> RICFNHQSSQPQTTKTCSPGES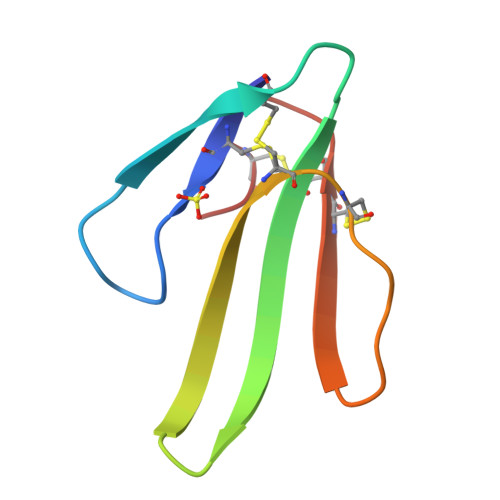SCYHKQWSDFRGTIIERGCGCPTVKPGIKLSCCESEVCNN> QLKLLVTRGKEQGYLTYAEVNDHLPEDIVDSDQIEDIIQMINDMGIQVMEEAPDADDLMLAENTADEDAAEAAAQVLSSVESEIGR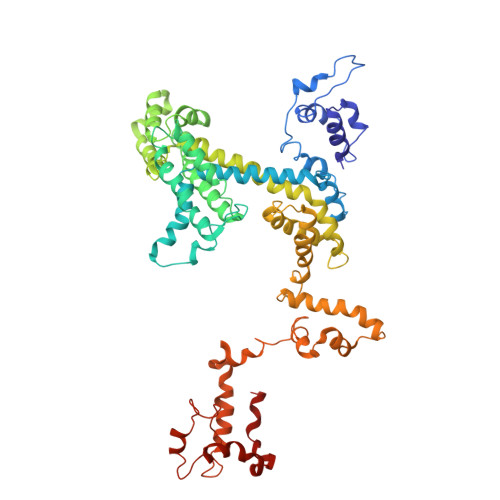TTDPVRMYMREMGTVELLTREGEIDIAKRIEDGINQVQCSVAEYPEAITYLLEQYDRVEAEEARLSDLITGFVDPNAENSIDPELAREKFAELRAQYVVTRDTIKAKGRSHATAQEEILKLSEVFKQFRLVPKQFDYLVNSMRVMMDRVRTQERLIMKLCVEQCKMPKKNFITLFTGNETSDTWFNAAIAMNKPWSEKLHDVSEEVHRALQKLQQIEEETGLTIEQVKDINRRMSIGEAKARRAKKEMVEANLRLVISIAKKYTNRGLQFLDLIQEGNIGLMKAVDKFEYRRGYKFSTYATWWIRQAITRSIADQARTIRIPVHMIETINKLNRISRQMLQEMGREPTPEELAERMLMPEDKIRKVLKISMETPIGDDEDSHLGIDFIEDTTSATTESLRAATHDVLAGLTAREAKVLRMRFGIDMNTDYTLEEVGKQFDVTRERIRQIEAKALRKLRHPSRSEVLRSFLDD>[2x]MKLALNTEFKKAIDLATNSSKNLFITGKAGTGKSTFLKYLINELLFDAVVLAPTGVAAINIGGETIHSFFNFPINITPDKIPDLFIYDYEIYKYVNTIIIDEISMVRADLLDCIDLFLKRVKNPKLPFGGTKMIFIGDLYQLPPVLTNHQKKAFNMEYESPYFFSAKVFKEMDMEFIEFETIYRQSDKLFIDILNRIRNNTVTDEDIKIINSRVQDKIDNDDGYIYITTVNKKAEEINNQKLDKLKGKLYKLNGTLKGNFDENSLPTPKNLHLKIGAQVMLLNNAPDRMWVNGTIGTITNIFPDEMIIELALENGNIVEITPFKWDMIKFTYDKKEKKMLSETIGSYTQFPLKLAYAITVHKSQGKTFHKVIIDTSRHFFAPGQFYVALSRCTSLDGIILTKKITKNSIILDKKVVNFLTNFQYQLSEKKTPLEEKISILKRAIERNSPLEIVYLKTKDEKSKRVIIPKEVGEMVYSGKSFMGLKGFCTMRNDERVFRIDRILEIKEIND

Pif1 is a DNA helicase belonging to family SF1B of Superfamily 1 (SF1), which unwinds dsDNA with 5′ to 3′ directionality. Pif1 is involved in DNA repair and is necessary for the maintenance of mitochondrial and nuclear genomes integrity, in the regulation of telomerase activity and in the replication fork progression. We were able to crystallize the helicase core of Pif1 from the thermophilic bacteria Deferribacter desulfuricans and Sulfurihydrogenibium sp., which are moderate thermophilic bacteria, living at an average temperature of 65 °C. Pif1 from these bacteria are named DdPif1 and SsPif1, respectively. The helicase core of Pif1 from thermophilic bacteria is very similar to other bacterial Pif1 structures already solved. The HC contains the features of previously described SF1B helicases: two RecA-like domains 1A and 2A containing insertions 1B and 2B, respectively.

DdPif1 apo crystallized in spacegroup C2221 with one molecule in the asymmetric unit and DdPif1 in the complex with the nucleotide analogue AMPPNP crystallized in spacegroup P21212 with two molecules in the asymmetric unit. Though solving this structure was not particularly difficult because of strong homology with the template structure BsPif1, used as a search model for MR, the DdPif1-AMPPNP structure has a possible domain swapping between the two molecules of the asymmetric unit. Indeed, the C-terminal half of the two Pif1 molecules, containing domains 2A and 2B, can be exchanged in a region where the electron density is ambiguous. However, we choose to consider the two molecules folded as compact structures with no swapped domains, since domain swapping of RecA domains in helicases was never reported before. Only one molecule of DdPif1 in the asymmetric unit is complexed with AMPPNP. The nucleotide has a good electron density which was also checked with the calculation of a simulated annealing omit map. The main difference is the folding of the N-terminal part of DdPif1 (residues 1-20). This N-terminal part is not visible in the DdPif1 structure and may be disordered. However, when AMPPNP is bound, the N-terminal part is visible and contributes to nucleotide binding. The adenine base is stacked by an aromatic residue of motif IV (Y183, Y186 or F187 in DdPif1, SsPif1, and BsPif1, respectively) and a hydrophobic site chain of a residue of the N-terminal tail (A4, V5 or M4 in DdPif1, SsPif1, and BsPif1, respectively).> ELTPDQQTLLHFIMDSYNKQRMPQEITNKILKEAFSAEENFLILTEMATNHVQVLVEFTKKLPGFQTLDHEDQIALLKGSAVEAMFLRSAEIFNKKLPSGHSDLLEERIRNSGISDEYITPMFSFYKSIGELKMTQEEYALLTAIVILSPDRQYIKDREAVEKLQEPLLDVLQKLCKIHQPENPQHFAKLLGRLTELRTFNHHHAEMLMSWRVDH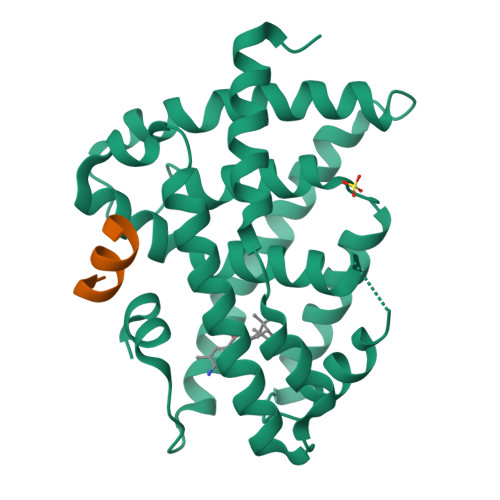KFTPLLQEIWDV;> EHQLLRYLLDK> LPRAKPLGEILVELGLARPED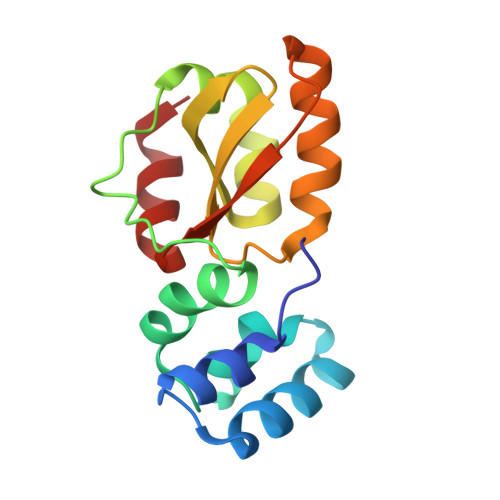VEEALQKQRRGGGRLEDTLVQSGKLRPEALAQAVATQLGYPYVDPEEDPPDPGAPLLLPEDLCRRYGVFPHRLEGNRLVLLMKDPRNILALDDVRLALKRKGLNYEVAPAVATEAAITKLIERFY> DAVVGSIAVPSVD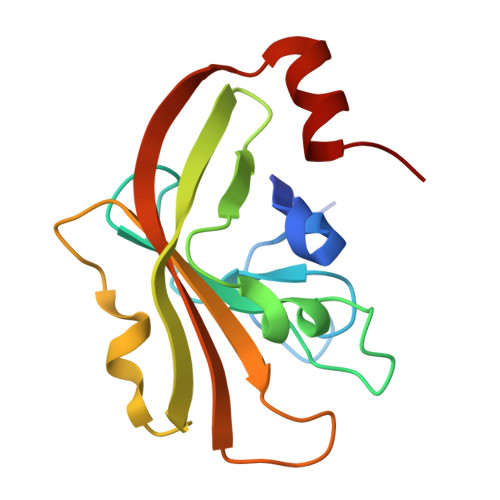VNLLVFKGTNTANLLAGATTMRSDQVMGKGNYPLAGHHMRDESMLFGPIMKVKKGDKIYLTDLENLYEYTVTETKTIDETEVSVIDNTKDARITLITCDKPTETTKRFVAVGELEKTEKLTKELENKYFPSK>[2x]MSTEASRSGKQEVDLTNCDREPIHIPGAIQPHGVLLVLSEPGLVLTHASENAPAVLGNSAEQLLGAPLGHFIEPSVREPLEADLRSARLKQLNPLKVVWRVDGVDRFFDGIAHRHQGRLILELEPSSHREAVPFLSFFHAVRDGLSRLRDARDLQELCEAVVQEVRGLTGFDRAIIYRFDAEWNGSVIAEARDARADPYLGLHFPASDIPRQARELYQLNWLRIIPTIDYQPARVRALPGHGEPLDLSFSVLRSVSPIHLEYLHNMGVQASMSISLMKDGKLWGLISCTQVSGTRYVPYEVRTACEFLGEVMSSLLAAKEGNEDYDQRIRAKSIHAALLERMAREVDFVSGLASQESGLLELVHAHGAAIHFHGRTTVLGQAPSDEALTGLIEWLGSRTGEGVFCTDRLAREYPEAQAFQEVAAGLMAFSMSRGRNNFVLWFRPEAVQTVNWSGNPTKAVEFDQGGPRLHPRKSFELWKETVRGRCLPWKAYEVE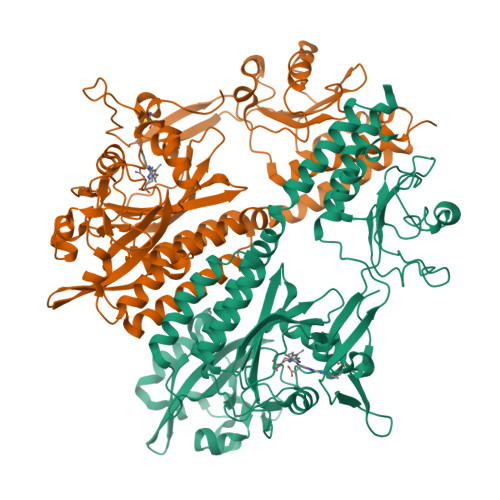AASELRRSIIDVALQRSE>MGGSHHHHHHGMASHKLLVTPPKALLKPLSIPNQLLLGPGPSNLPPRIMAAGGLQMIGSMSKDMYQIMDEIKEGIQYVFQTRNPLTLVISGSGHCALEAALVNVLEPGDSFLVGANGIWGQRAVDIGERIGARVHPMTKDPGGHYTLQEVEEGLAQHKPVLLFLTHGESSTGVLQPLDGFGELCHRYKCLLLVNSVASLGGTPLYMDRQGIDILYSGSQKALNAPPGTSLISFSDKAKKKMYSRKTKPFSFYLDIKWLANFWGCDDQPRMYHHTIPVISLYSLRESLALIAEQGLENSWRQHREAAAYLHGRLQALGLQLFVKDPALRLPTVTT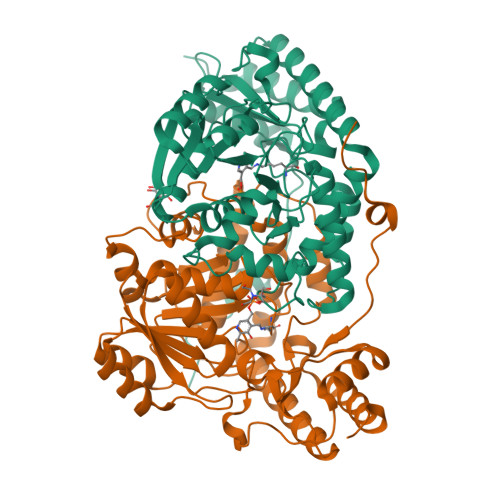VAVPAGYDWRDIVSYVIDHFDIEIMGGLGPSTGKVLRIGLLGCNATRENVDRVTEALRAALQHCPKKKL[8x]Strept­avidin, a 52.8 kDa protein (four monomers in the asymmetric unit) from S. avidinii, is one of these cases: this 508-residue tetrameric protein has no sulfur-containing residues nor any other significant anomalous scatterers. However, each monomer unit of strept­avidin strongly binds one molecule of biotin, a sulfur-containing ligand. In fact, the strept­avidin–biotin interaction is one of the strongest non­covalent interactions known in biology, and this turned out to be advantageous for substructure determination.

Native SAD can be a successful method even in particularly difficult cases where few anomalous scatterers are present. The strept­avidin–biotin complex has a Bijvoet ratio of 0.6% at 6 keV, one of the lowest yet tested, and crystallizes in the monoclinic space group P21. Using the low-dose, multi-orientation method described above, a total of 5040° (14 × 360°) of data were collected from a large (50 × 150 × 200 µm) single crystal of strept­avidin–biotin over two different areas of the crystal and at varying orientations. At 6 keV energy and a sample-to-detector distance of 120 mm, the resolution of the native SAD data collected was 2.1 Å. The phase-extended map was used for model building with ARP/wARP, and refinement with phenix.refine proceeded smoothly thereafter. Phase extension was not strictly necessary to finish the model building and refinement, but rather to show the utility of combining the low-energy SAD data with data collected at a higher energy to improve the resolution.

>AEAGITGTWYNQLGSTFIVTAGADGALTGTYESAVGNAESRYVLTGRYDSAPATDGSGTALGWTVAWKNNYRNAHSATTWSGQYVGGAEARINTQWLLTSGTTEANAWKSTLVGHDTFTKVKPSAAS[4x]> MGSENIYTTLKFESMMQQRVIQIRSIPEEEYHELVSVQGDGDGPIQVSVFVQSAAKVFTEFEQGCDTIGRSKVESIYLYKFNLLQTAFFAMVSEKVNDWTQLYKDVRYLYTENPKLLQLMELNSRRLDLNLNLIKKTIYKLVNDQLQELKDNERTPDWD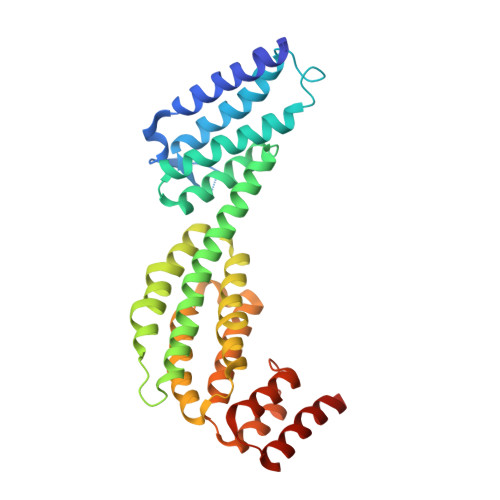ITISSLLPYLKKTALPTLYKLEDNTILVALIRYIVHDLVIDNILHWRVISEKSSENLSEFIMLLLSGLEIPRLNLIETYRHSREKLGILSKILTAHLKDILEMFYEGEFFLFETDEIVQWIILLFADTPTRRDCIDEIRRVREEATD>RTKDKYRVVYTDHQRLELEKEFHYSRYITIRRKAELAATLGLSERQVKIWFQNRRAKERKINKKKLQQQQQQ[2x]

To elucidate the mechanism, we performed structural analysis of two homeodomain proteins, the posterior homeodomain protein HOXB13, and the parahox protein CDX2, each bound to two distinct high-affinity sequences. The optimal sequences for HOXB13 are CCAATAAA and CTCGTAAA that differ from each other by the three underlined base pairs, whereas CDX2 binds with high affinity to similar two sequences that begin with a G instead of a C. Two parts of both HOXB13 and CDX2 DBDs interact with DNA: the recognition helix α3, which tightly packs into the major groove, and the N-terminal tail interacting with the minor groove. Instead, thermodynamic analyses of HOXB13, CDX2, BARHL2 and MYF5 revealed that the two optimal states were bound because of their distinct effects on enthalpy and entropy, principally caused by differential stability of the water network at the protein-DNA interface.

The overall protein structure in the four complexes is highly similar, showing only minor differences in the conformation of the N-termini, due to the replacement of basic Arg-217 of HOXB13 with the negatively charged Asp-187 in CDX2. The corresponding contact (Arg-228 to backbone) is also observed in both CDX2 structures. In CDX2 complexes the DNA bend in CDX2-DNATCG is slightly smaller due to the replacement of Thr-261 with Lys-231 which does not allow the alternative conformation of Arg-228. Consistently, only few water molecules were found in the CDX2-DNATCG complex. In complex of CDX2-DNATCG with high resolution (2.57 Å) the water molecules were well visible but they did not form the corresponding water-chains supporting the idea of entropically driven binding. The channel is not as clearly visible from one side of the CDX2-DNATCG complex because of the presence of Lys-231 instead of Thr-261. The long side chain of Lys-231 does not allow Arg-228 (corresponded to Arg-258 in HOXB13) to change its conformation easily. Together, Arg-228 and Lys-231 close the entry of the channel from this side but the other end of the channel is open and well visible in CDX2-DNATCG. Similarly, the two CDX2-DNA structures also displayed very similar overall conformations.> MGSDKIHHHHHHENLYFQGMTTSKVTYQGDLRTSAIHLQSNNEIITDAPVDNQGKGEAFSPTDLLATSLASCMLTIIGIKARDMEIDIAGTTAEVTKVMAADPRRVSEVHIAITFNQELDDKTQKIFYNTALTCPVAKSIHPDIFQK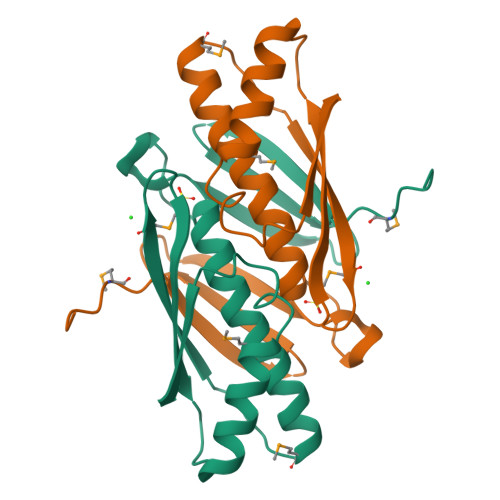VIIHSKSY> SANNPWTGFQIFLSPYYANEVAAAAKQITDPTLSSKAASVANIPTFTWLDSVAKIPDLGTYLASASALGKSTGTKQLVQIVIYDLPDRDCAAKASNGEFSIANNGQANYENYIDQIVAQIQQFPDVRVVAVIEPDSLANLVTNLNVQKCANAKTTYLACVNYALTNLAKVGVYMYMDAGHAGWLGWPANLSPAAQLFTQVWQNAGKSPFIKGLATNVANYNALQAASPDPITQGNPNYDEIHYINALAPLLQQAGWDATFIVDQGRSGVQNIRQQWGDWCNIKGAGFGTRPTTNTGSQFIDSIVWVKPGGECDGTSNSSSPRYDSTCSLPDAAQPAPEAGTWFQAYFQTLVSAANPPL

Cellobiohydrolases (EC 3.2.1.91), which hydrolyze cellulose to cellobiose (a β-1,4-linked d-glucose dimer), are key members of their enzyme cocktails, playing a major role in the hydrolysis of crystalline cellulose. The GH family 6 cellobiohydrolase from the basidiomycete P. chrysosporium (PcCel6A) consists of a catalytic domain (CD) and an N-terminal carbohydrate-binding module (CBM) connected by a linker region; this modular structure is typical of fungal GH family 6 cellobiohydrolases. The final structures included residues 82–439. The catalytic site is located in a tunnel enclosed by a pair of loops (residues 174–178 and 390–425), designated here as the N-terminal and C-terminal loops.

X-ray data sets were collected from a PcCel6A crystal and a pNPG3-soaked crystal to 1.2 and 2.1 Å resolution, respectively. Two major conformations of the loops are known, an ‘open’ conformation that makes the subsites more accessible and a ‘closed’ conformation for arrangement of the catalytic site residues into the catalytically competent configuration. In the cellobiose-bound structure, the loops adopted the closed conformation, in contrast to the open conformation observed in the apo structure. The residues in the loops have consistently high B factors compared with other regions of the protein. As shown in Fig. 4(a), the N- and C-terminal loops of the PcCel6A apo structure were both modelled as double conformations with similar occupancies ranging from 0.46 to 0.54. In §3.2, the loops of PcCel6A remained open in the absence of bound ligand, but occupation of the substrate-binding sites induced conformational change of the loops, resulting in a narrowing of the active-site cleft. In the C-terminal loop region, on the other hand, the r.m.s.d. values between the apo and cellobiose-bound structures were similar to that between the two conformations of the apo structure. Therefore, both loops showed clear flexibility, but their mobility and response to ligand binding were different.>GSMELRVGNKYRLGRKIGSGSFGDIYLGANIASGEEVAIKLECVKTKHPQLHIESKFYKMMQGGVGIPSIKWCGAEGDYNVMVMELLGPSLEDLFNFCSRKFSLKTVLLLADQMISRIEYIHSKNFIHRDVKP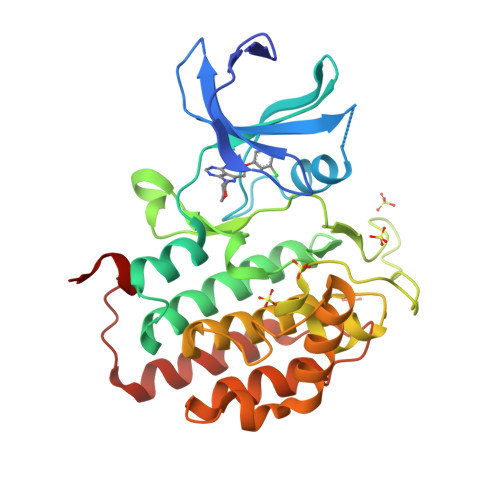DNFLMGLGKKGNLVYIIDFGLAKKYRDARTHQHIPYRENKNLTGTARYASINTHLGIEQSRRDDLESLGYVLMYFNLGSLPWQGLKAATKRQKYERISEKKMSTPIEVLCKGYPSEFSTYLNFCRSLRFDDKPDYSYLRQLFRNLFHRQGFSYDYVFDWNMLK[2x]> MEGERKNNNKRWYFTREQLENSPSRRFGVDPDKELSYRQQAANLLQDMGQRLNVSQLTINTAIVYMHRFYMIQSFTRF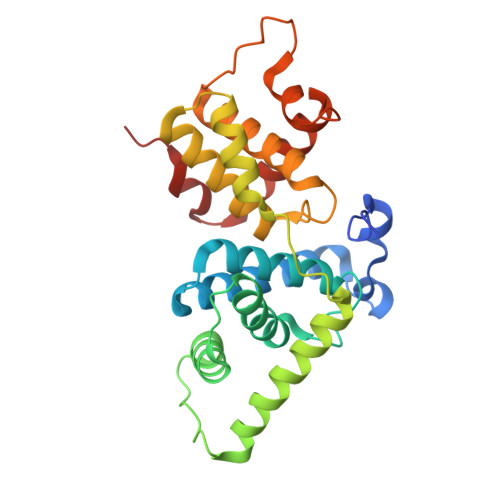PGNSVAPAALFLAAKVEGQPKKLEHVIKVAHTCLHPQESLPDTRSEAYLQQVQDLVILESIILQTLGFELTIDHPHTHVVKCTQLVRASKDLAQTSYFMATNSLHLTTFSLQYTPPVVACVCIHLACKWSNWEIPVSTDGKHWWEYVDATVTLELLDELTHELLQILEKTPNRLKRIWNWR>GGGAAAUGAUGGGCGUAGACGCACGUCAGCGGCGGAAAUGGUUUCCC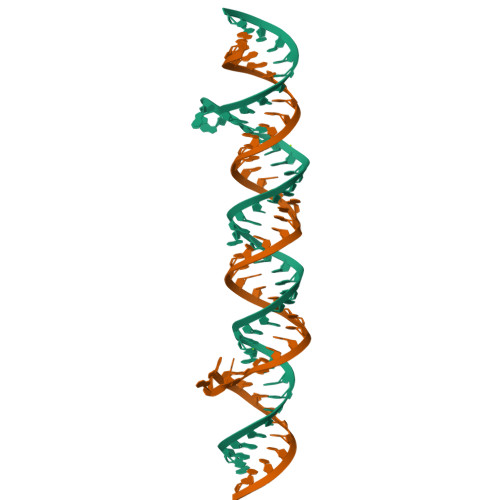[2x]>[3x]MKKIIETQRAPGAIGPYVQGVDLGSMVFTSGQIPVCPQTGEIPADVQDQARLSLENVKAIVVAAGLSVGDIIKMTVFITDLNDFATINEVYKQFFDEHQATYPTRSCVQVARLPKDVKLEIEAIAVRSA

The sixth gene of the tdc operon encodes a protein, TdcF, that is a member of the YjgF/YER057c/UK114 family. The location of this gene within the tdc operon is strongly suggestive of a role in the degradation of 2-ketobutyrate. Each 14 kDa subunit comprises a single domain that contains a predominantly anti-parallel, six-stranded β-sheet against which are packed two short α-helices. The most significant structural features are the three symmetry-related solvent-accessible clefts, located at the interfaces between pair of subunits, close to the "equator" of the trimer.

The first crystal structure of TdcF was determined at 2.35 Å resolution by molecular replacement using the structure of the paralogue YjgF as a template. The original 2.35 Å resolution as-isolated X-ray data set was collected at 100 K using a cryoprotectant solution containing 20% (v/v) ethylene glycol. During model building and refinement, it became apparent that whilst the electron density in site A was consistent with ordered water molecules, a more substantial region of elongated density was present in both sites B and C. This could be modelled convincingly as a single ethylene glycol molecule in each of the two sites making a single hydrogen bonding interaction with the side chain of Arg-105. It was noted that the central part of the loop connecting β1 and β2, which delineates one side of the cleft and bears the conserved residue Tyr-17, had elevated temperature factors, with Ile-14 being poorly defined in the electron density maps. Since ethylene glycol makes only a single hydrogen bond with TdcF, it is likely that it binds with low affinity, and it is only seen in the structure because of its high concentration in the cryoprotectant. In our initial structure of TdcF, the cryoprotectant ethylene glycol was shown to occupy two of the three binding sites, but this is unlikely to be physiologically relevant.> MSSSVCPSDNTHATGAALQKILDYKKGDHQIMAGYFRSWRDTASGTGNKVSMLDLPDCLDIAFVFPEGDETASFWTTLKDTYVPALHGRGIKVVRSVGIAQLINTAWDNTPAGWQGLADALMKTVDDYGLDGLDINVQQSLNANQLKQATGVFNALAKKLGPKSGTGKLLIFDTNMDGTQPLWRNVYPTISYVL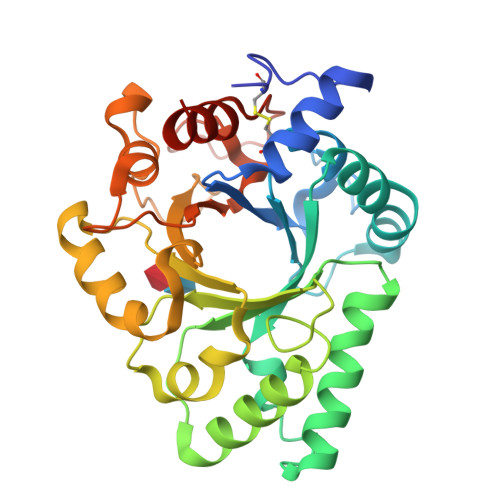IQSYGRSISGLQTTYNSFKSYISSKQYLIGFSFYEENGTNWGDTTTPMTSSRAWQYAKWQPSGATKGGIFSYAIDRDGVAIGDNTLKTTDFTWTRQLIGAMNPHHHHHH> GSMKKVEAIIRPEKLEIVKKALSDAGYVGMTVSEVKGRGVQGG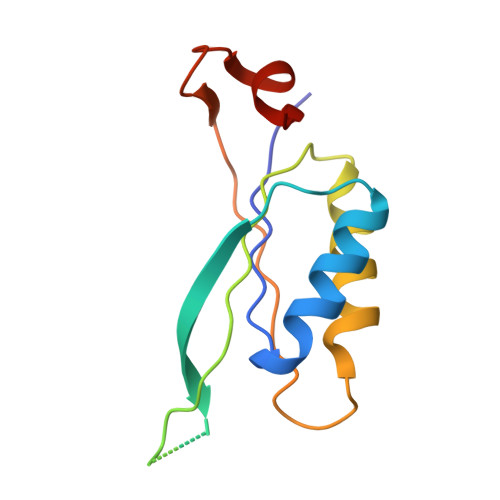IVERYRGREYIVDLIPKVKIELVVKEEDVDNVIDIICENARTGNPGDGKIFVIPVERVVRVRTKEEGKEALLEHHH> NAQYHL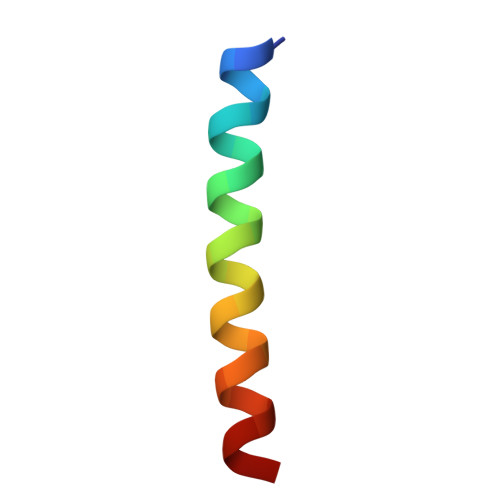LVKQGDGLLTKLQKYGAAVR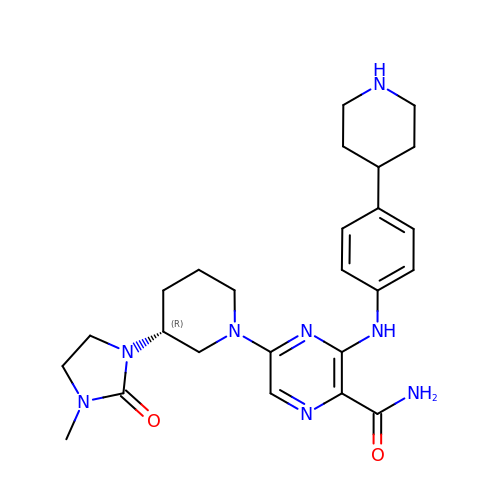5-[(3R)-3-(3-methyl-2-oxoimidazolidin-1-yl)piperidin-1-yl]-3-[4-(piperidin-4-yl)anilino]pyrazine-2-carboxamide | C25 H34 N8 O2 | JCGXVYWABUYORV-HXUWFJFHSA-N>[2x]GASHPVVTEVIIPENPR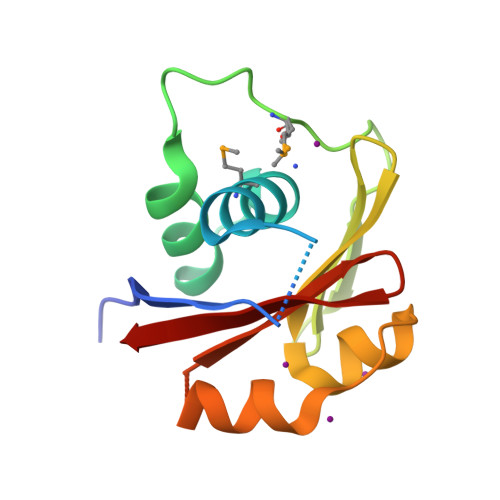HNLNDTWSEVEVLMLAAAVESNTTHPVGKAIVKAARARNCQTMKAEDGTFTEEPGSGAVAIVNNKRVTVGTLEWVKRHGATGNSLLALAAHEINNQSVVYIGVDNTLAAVIRFE>[2x]MTTNYIFVTGGVVSSLGKGIAAASLAAILEARGLNVTIMKLDPYINVDPGTMSPIQHGEVFVTEDGAETDLDLGHYERFIRTKMSRRNNFTTGRIYSDVLRKERRGDYLGATVQVIPHITNAIKERVLEGGEGHDVVLVEIGGTVGDIESLPFLEAIRQMAVEIGREHTLFMHLTLVPYMAASGEVKTKPTQHSVKELLSIGIQPDILICRSDRAVPANERAKIALFCNVPEKAVISLKDVDSIYKIPGLLKSQGLDDYICKR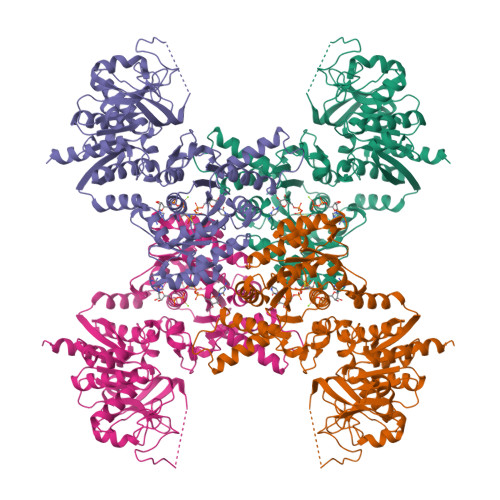FSLNCPEANLSEWEQVIFEEANPVSEVTIGMVGKYIELPDAYKSVIEALKHGGLKNRVSVNIKLIDSQDVETRGVEILKGLDAILVPGGFGYRGVEGMITTARFARENNIPYLGICLGMQVALIDYARHVANMENANSTEFVPDCKYPVVALITEWRDENGNVEVRSEKSDLGGTMRLGAQQCQLVDDSLVRQLYNAPTIVERHRHRYEVNNMLLKQIEDAGLRVAGRSGDDQLVEIIEVPNHPWFVACQFHPEFTSTPRDGHPLFAGFVKAASEFQKRQAK> PIVEIHLLEGYSDAEKERLGRSLTAAVQTVVPAPPEAITVMMHEMQAADYMRGATRRTPAPALPDAAATVRDFLDT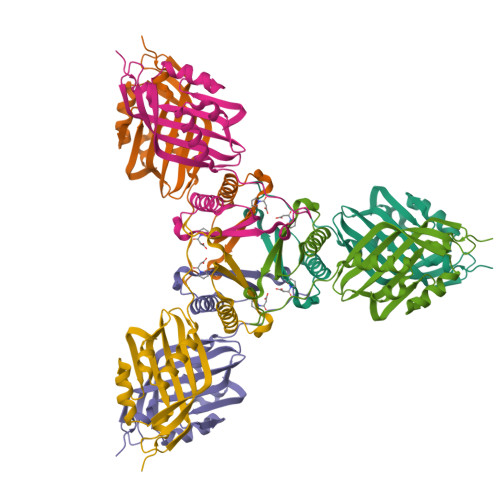MEARDLDKARTFLTDDFVMTFPTGRRMTDLSDLVEWSATRYRFVTKTYDRFDTAATLDGPVVYCFGTLRGEWPDGTPFDNVRFIDRFALRDGKLAVQDVWNDLEAMRPRG> GAMGSSEAQTTDSDDVIVPPMSQKYPKADSEKMCIEIVSLAFYPEAEVMSDENIKQVYVEYKFYDLPLSETETPVSLRKPRAGEEIHFHFSKVIDLDPQEQQGRRRFLFDMLNGQDPDQGHLKFTVVSDPLDEEKKECEEVGYAYLQLWQILESGRDILEQELDIVSPEDLATPIGRLKVSLQAAAVLHAIYKEMTE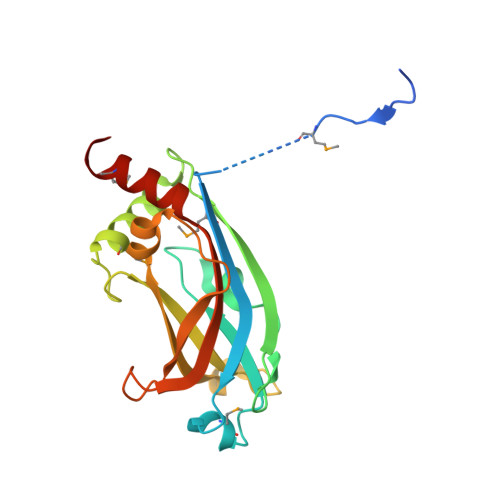DLFS> SNAMRGYYDEISFDVNTTAKKMHLFLMRSIASYDVTPEQWSVLEGIEANEPISQKEIALWTKKDTPTVNRIVDVLLRKELIVREISTEDRRISLLSLTDKGRKETTELRDIVEASCEKM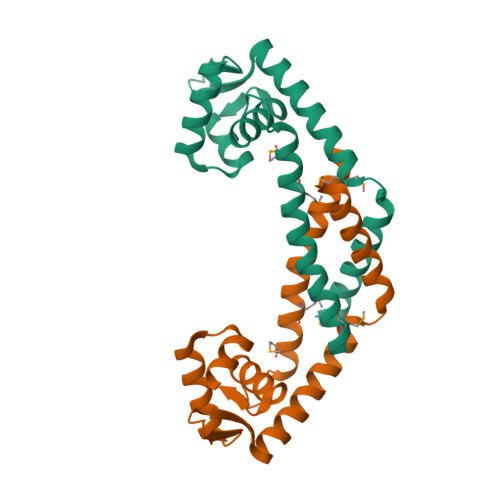FAGVTRTDLEQFTAILKNISTNIE Bile salt hydrolases (BSHs) catalyze the amino acid deconjugation reactions required to liberate free bile acids for subsequent and successive modifications and metabolism. The BSHs belong to the N-terminal nucleophile hydrolase (Ntn-hydrolase) superfamily, which is characterized by an αββα core structure that is subject to autoactivation. Here, we identify and describe the BSH from a common member of the Plains bison microbiome, Arthrobacter citreus (BSHAc). Steady-state kinetic analyses demonstrated that BSHAc is a broad-spectrum hydrolase with a preference for glycine-conjugates and deoxycholic acid (DCA).

To assess conserved and divergent structure-function relationships between BSHAc and other BSHs, we crystallized the enzyme and obtained a three-dimensional structure using X-ray diffraction data. A model of BSHAc was refined at a resolution 2.0 Å. It showed the typical αββα-sandwich architecture and autoactivated N-terminal catalytic Cys (Cys2) nucleophile of the BSHs. The asymmetric unit of the BSHAc crystals contained a dimer. The protomers of this dimer are arranged in such a manner that part of the substrate binding site – the amino acid-binding region – is shaped by both protomers. In BSHAc, a 36-amino acid loop extending from α3 and terminating in α4 contains a β-sheet as well as a proposed substrate selectivity motif. The latter participates in the formation of a dimer-dependent substrate-binding site with the loop swapped between the two protomers. At a higher level, this dimer-swapped (DS) loop also contributes to the tetrameric biological assembly of BSHAc. In BSHAc, the interface between the loop-swapped dimers covers an area of ∼2100 Å2 whereas the total area of interaction between protomers in the tetramer is ∼7200 Å2. In the inhibitor-free BSHAc, residues Trp22 and Phe26 appear in a T-shaped π-stacking arrangement whereas the presence of the inhibitor alters their interaction.

>[2x]CTGIRYSDGSGNLYLARNLDWTSDFGERVVVTPTGYTTKSPFGAVPAIRHAVIGMGIVQEDTPLYFDCGNDAGLAVAGLNFPGYAQYATEAVDGATNVAAFEFPLWVASQFASVDEVEAALADVVIVDRPINDKYPSSLLHWIIGDSKRAIVVEYTSDGLHVFDDDVDVLANQPGFGWHHENLRNYLNASPDFPEKIVLNRADLVPFGSGSLMRGIPGDYYSPSRFVRAAYVHAHYPGKSTEEENVSRAFHTLQQVAMVDGSAAMGSGEFEKTTYTGLFSSRTMTYYWNTYEDPAVRSVAMADHAADGTELVVVLEHHHHHH Gastric infection by H. pylori depends on the expression of a nickel-dependent urease in the cytoplasm of the bacteria. The ure gene cluster is comprises seven genes, two of which code for a nickel-dependent urease (ureA and ureB) that hydrolyzes urea into NH3 and CO2, one for a pH-gated urea channel (ureI) that delivers host gastric urea to urease in the bacterial cytoplasm, and four for cytoplasmic accessory proteins involved in nickel processing. Ureases (EC 3.5.1.5) are amidohydrolases found in bacteria, algae, plants and fungi with an active site composed of a carbamylated lysine (KCX)14 coordinating a bi-nickel center. The overall single-particle cryo-EM structures of H. pylori urease reveal a 1.1 MDa dodecameric complex of 12 UreA and 12 UreB subunits in a tetrahedral arrangement, in agreement with the previously published crystal structures.

The map at 2.5 Å resolution depicts urease with BME bound in the active site (U-BME) whereas the map at 2.0 Å details the binding of an inhibitor 2-{[1-(3,5-dimethylphenyl)-1H-imidazol-2-yl]sulfanyl}-N-hydroxyacetamide (U-SHA). We determined urease IC50 values under identical conditions for BME and SHA as 13.5 mM and 19.6 μM, respectively. The density for SHA shows that its hydroxamic acid moiety interacts with both active site Ni+2 while its rings interact with the UreB flap region. SHA coordinates with the bi-nickel center through its hydroxamic acid hydroxyl O18 with distances of 1.98 and 3.10 Å. In addition, SHA O18 accepts a 3.06 Å hydrogen bond from His221 Nε2. Further away from the hydroxamic acid moiety, van der Waals interactions occur between the imidazole and phenyl rings of the inhibitor and flap region residues, especially conserved residues Cys321 and His322 whose side chains are within 3.5 Å of SHA. The difference in flap region positioning appears to be due to the bulky SHA imidazole and phenyl rings that would sterically clash with the side chains of Cys321 and His322 at the tip of the flap in the BME complex, with both residues fully conserved for the 260 GenBank deposited H. pylori urease sequences. This steric hindrance results in a displacement of the flap residues away from the active site, with residues UreB B321-324 having RMSD values close to 2.0 Å. Interestingly, despite the binding of a bulky inhibitor the conformation of the active site residues and the coordination between the active site residues and the bi-Ni center is not disturbed when compared to U-BME and to the previously published U-NAT and U-AHA crystal structures.

>[12x]MKLTPKELDKLMLHYAGELARKRKEKGIKLNYVEAVALISAHIMEEARAGKKTAAELMQEGRTLLKPDDVMDGVASMIHEVGIEAMFPDGTKLVTVHTPIEANGKLVPGELFLKNEDITINEGKKAVSVKVKNVGDRPVQIGSHFHFFEVNRCLDFDREKTFGKRLDIASGTAVRFEPGEEKSVELIDIGGNRRIFGFNALVDRQADNESKKIALHRAKERGFHGTKSDDNYVKTIKE;>MKKISRKEYVSMYGPTTGDKVRLGDTDLIAEVEHDYTIYGEELKFGGGKTLREGMSQSNNPSKEELDLIITNALIVDYTGIYKADIGIKDGKIAGIGKGGNKDMQDGVKNNLSVGPATEALAGEGLIVTAGGIDTHIHFISPQQIPTAFASGVTTMIGGGTGPADGTNATTITPGRRNLKWMLRAAEEYSMNLGFLAKGNTSNDASLADQIEAGAIGFKIHEDWGTTPSAINHALDVADKYDVQVAIHTDTLNEAGCVEDTMAAIAGRTMHTFHTEGAGGGHAPDIIKVAGEHNILPASTNPTIPFTVNTEAEHMDMLMVCHHLDKSIKEDVQFADSRIRPQTIAAEDTLHDMGIFSITSSDSQAMGRVGEVITRTWQTADKNKKEFGRLKEEKGDNDNFRIKRYLSKYTINPAIAHGISEYVGSVEVGKVADLVLWSPAFFGVKPNMIIKGGFIALSQMGDANASIPTPQPVYYREMFAHHGKAKYDANITFVSQAAYDKGIKEELGLERQVLPVKNCRNITKKDMQFNDTTAHIEVNPETYHVFVDGKEVTSKPANKVSLAQLFSIF[12x]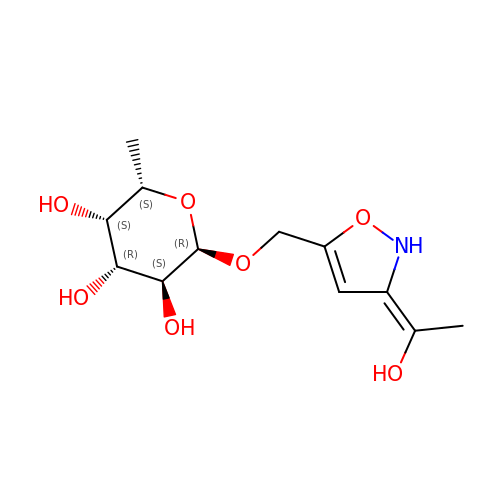[(3E)-3-(1-hydroxyethylidene)-2,3-dihydroisoxazol-5-yl]methyl alpha-L-fucopyranoside | C12 H19 N O7 | DQRDRRBASDQFKR-AWJQDWPASA-N>[11x]MAALIAENFRFLSLFFKSKDVMIFNGLVALGTVGSQELFSVVAFHCPCSPARNYLYGLAAIGVPALVLFIIGIILNNHTWNLVAECQHRRTKNCSAAPTFLLLSSILGRAAVAPVTWSVISLLRGEAYVCALSEFVDPSSLTAREEHFPSAHATEILARFPCKENPDNLSDFREEVSRRLRYESQLFGWLLIGVVAILVFLTKCLKHYCS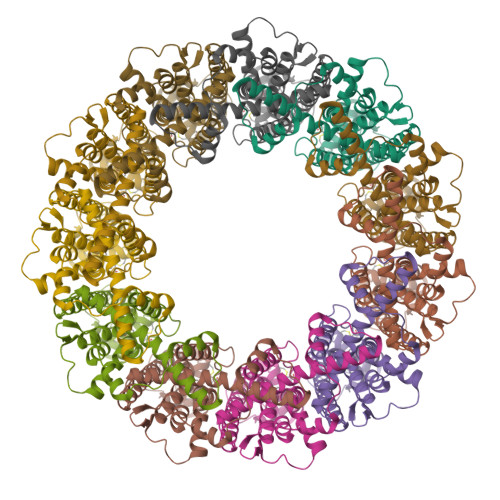PLSYRQEAYWAQYRANEDQLFQRTAEVHSRVLAANNVRRFFGFVALNKDDEELIANFPVEGTQPRPQWNAITGVYLYRENQGLPLYSRLHKWAQGLAGNGAAPDNVEMALLPSFESRLVPR Plasma membrane Ca2+-ATPases (PMCAs) have a crucial role in this process by extruding Ca2+ against a steep concentration gradient from the cytosol to the extracellular space. Native PMCAs form heterodimeric assemblies with the small transmembrane proteins neuroplastin (NPTN) and basigin (BASI). Here we present the structures of mouse PMCA2 in the presence and absence of its accessory subunit neuroplastin in eight different stages of its transport cycle. The structures revealed an overall classical P-type ATPase architecture with ten transmembrane helices characteristic of the P2 subgroup.

We first expressed mouse PMCA2 in NPTN/BSG-knockout cells (BSG encodes BASI) to obtain a homogeneous population of target protein for structural analyses, enabling us to isolate PMCA2 both alone and exclusively complexed with NPTN when the latter was co-expressed. Moreover, solitary PMCA2 structures obtained from an NPTN-free environment in both the ion-bound E1-Ca-ATP state and the ion-free E2P state were indistinguishable from PMCA2 co-assembled with NPTN. In line with our structural findings, these results indicate that NPTN does not directly impact the transport activity of PMCA2. For a better understanding of the PMCA Ca2+ transport mechanism, we analysed Ca2+ binding in the E1-Ca and E1-Ca-ATP structures. We identified only one binding site formed by the backbones of residues V407, V408 and V410 and the side chains of residues E412, N869 and D873. This binding site is equivalent to site II of the two Ca2+-binding sites of SERCA.

> MGDMTNSDFYSKNQRNESSHGGEFGCTMEELRSLMELRGTEAVVKIKETYGDTEAICRRLKTSPVEGLPGTAPDLEKRKQIFGQNFIPPKKPKTFLQLVWEALQDVTLIILEIAAIISLGLSFYHPPGESNEGCATAQGGAEDEGEAEAGWIEGAAILLSVICVVLVTAFNDWSKEKQFRGLQSRIEQEQKFTVVRAGQVVQIPVAEIVVGDIAQIKYGDLLPADGLFIQGNDLKIDESSLTGESDQVRKSVDKDPMLLSGTHVMEGSGRMVVTAVGVNSQTGIIFTLLGAGGEEEEKKDKKAKQQDGAAAMEMQPLKSAEGGDADDKKKANMHKKEKSVLQGKLTKLAVQIGKAGLVMSAITVIILVLYFTVDTFVVNKKPWLTECTPVYVQYFVKFFIIGVTVLVVAVPEGLPLAVTISLAYSVKKMMKDNNLVRHLDACETMGNATAICSDKTGTLTTNRMTVVQAYVGDVHYKEIPDPSSINAKTLELLVNAIAINSAYTTKILPPEKEGALPRQVGNKTECGLLGFVLDLRQDYEPVRSQMPEEKLYKVYTFNSVRKSMSTVIKMPDESFRMYSKGASEIVLKKCCKILSGAGEARVFRPRDRDEMVKKVIEPMACDGLRTICVAYRDFPSSPEPDWDNENDILNELTCICVVGIEDPVRPEVPEAIRKCQRAGITVRMVTGDNINTARAIAIKCGIIHPGEDFLCLEGKEFNRRIRNEKGEIEQERIDKIWPKLRVLARSSPTDKHTLVKGIIDSTHTEQRQVVAVTGDGTNDGPALKKADVGFAMGIAGTDVAKEASDIILTDDNFSSIVKAVMWGRNVYDSISKFLQFQLTVNVVAVIVAFTGACITQDSPLKAVQMLWVNLIMDTFASLALATEPPTETLLLRKPYGRNKPLISRTMMKNILGHAVYQLTLIFTLLFVGEKMFQIDSGRNAPLHSPPSEHYTIIFNTFVMMQLFNEINARKIHGERNVFDGIFRNPIFCTIVLGTFAIQIVIVQFGGKPFSCSPLQLDQWMWCIFIGLGELVWGQVIATIPTSRLKFLKEAGRLTQKEEIPEEELNEDVEEIDHAERELRRGQILWFRGLNRIQTQIRVVKAFRSSLYEGLEKPESRTSIHNFMAHPEFRIEDSQPHIPLIDDTDLEEDAALKQNSSPPSSLNKNNSAIDSGINLTTDTSKSATSSSPGSPIHSLETSLENLYFQGGDYKDDDDK> MGNICVGGSRMAHQVNSPDRVSNNSGDEDNVTSSQL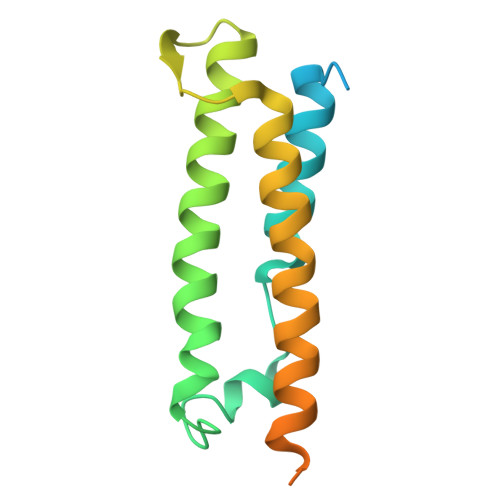LSVRHQLAESAGLPRDQHEFVSSQAPQSLRNRYNNLYSHTQRTLDMADMQHRYMTGASGINPGMLPHENVDDMRSAITDWSDMREALQHAMGIHADIPPSPERFVATMNPSGSIRMSTLSPSPYRNWQ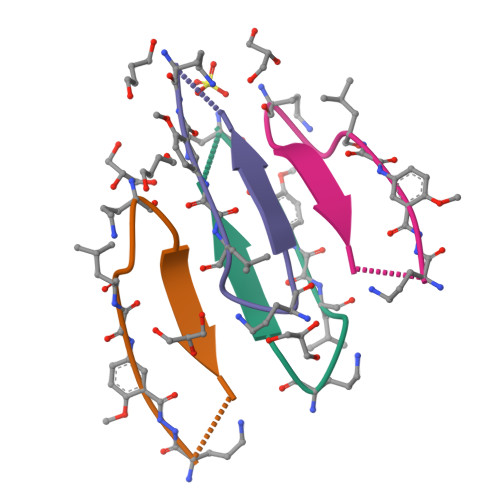>[8x]LVFFAAXLKA(3R)-3-benzyl-4-oxo-4-[(2-oxo-2-phenylethyl)sulfanyl]butanoic acid | C19 H18 O4 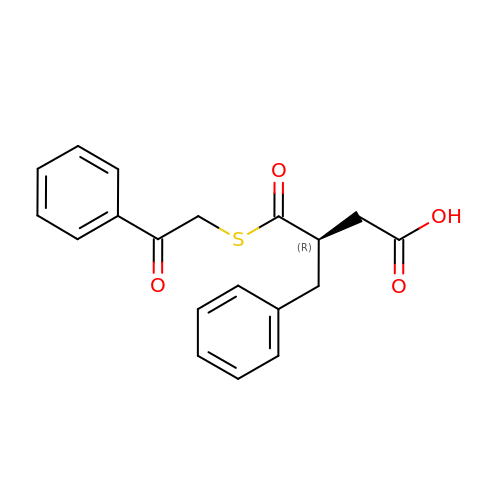S | XBDWLLDIBQGWMW-MRXNPFEDSA-N>GAMVRRSFSDEEGSSEDLLELSDVDSESSDISQPYVVCRQCPEYRRQAAQPPHCPAPEGEPGAPQALGDAPSTSVSLTTAVQDYVCPLQGSHALCTCCFQPMPDRRVEREQDPRVAPQQCAVCLQPFCHLYWGCTRTGCYGCLAPFCELNLGDKCLDGVLNNNSYESDILKNYLATRGLTWKNMLTESLVALQRGVFLLSDYRVTGDTVLCYCCGLRSFRELTYQYRQNIPASELPVAVTSRPDCYWGRNCRTQVKAHHAMKFNHICEQTRFKN[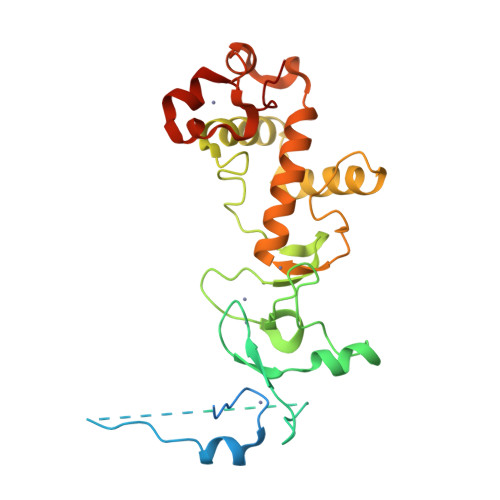2x]>GPGHMEASPASGPRHLMDPHIFTSNFNNGIGRHKTYLCYEVERLDNGTSVKMDQHRGFLHNQAKNLLCGFYGRHAALRFLDLVPSLQLDPAQIYRVT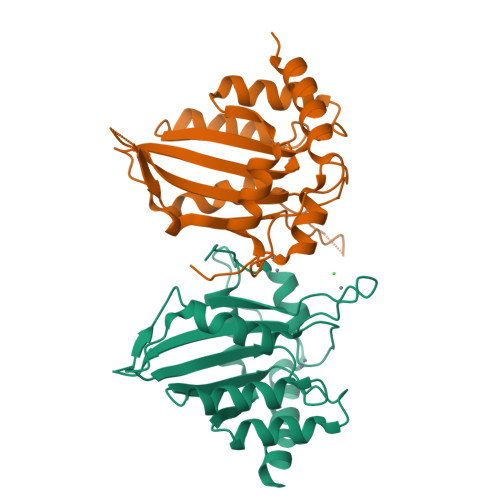WFISWSPCFSWGCAGEVRAFLQENTHVRLRIFAARIYDYDPLYKEALQMLRDAGAQVSIMTYDEFKHCWDTFVDHQGAPFQPWDGLDEHSQALSGRLRAILQNQGN[2x]>DLSSLTPGGSMGLQVNRGSQSSLEGAPATAPEPHSLGILHASYSVSHRVRPWWDITSCRQQWTRQILKDVSLYVESGQIMCILGSSGSGKTTLLDAMSGRLGRAGTFLGEVYVNGRALRREQFQDCFSYVLQSDTLLSSLTVRETLHYTALLAIRRGNPGSFQKKVEAVMAELSLSHVADRLIGNYSLGGISTGERRRVSIAAQLLQDPKVMLFDEPTTGLDCMTANQIVVLLVELARRNRIVVLTIHQPRSELFQLFDKIAILSFGELIFCGTPAEMLDFFNDCGYPCPEHSNPFDFYMDLTSVDTQSKEREIETSKRVQMIESAYKKSAICHKTLKNIERMKHLKTLPMVPFKTKDSPGVFSKLGVLLRRVTRNLVRNKLAVITRLLQNLIMGLFLLFFVLRVRSNVLKGAIQDRVGLLYQFVGATPYTGMLNAVNLFPVLRAVSDQESQDGLYQKWQMMLAYALHVLPFSVVATMIFSSVCYWTLGLHPEVARFGYFSAALLAPHLIGEFLTLVLLGIVQNPNIVNSVVALLSIAGVLVGSGFLRNIQEMPIPFKIISYFTFQKYCSEILVVNEFYGLNFTCGSSNVSVTTNPMCAFTQGIQFIEKTCPGATSRFTMNFLILYSFIPALVILGIVVFKIRDHLISRGSHHHHHHGHHHHHH[2x];>MGSAGKAAEERGLPKGATPQDTSGLQDRLFSSESDNSLYFTYSGQPNTLEVRDLNYQVDLASQVPWFEQLAQFKMPWTSPSCQNSCELGIQNLSFKVRSGQMLAIIGSSGCGRASLLDVITGRGHGGKIKSGQIWINGQPSSPQLVRKCVAHVRQHNQLLPNLTVRETLAFIAQMRLPRTFSQAQRDKRVEDVIAELRLRQCADTRVGNMYVRGLSGGERRRVSIGVQLLWNPGILILDEPTSGLDSFTAHNLVKTLSRLAKGN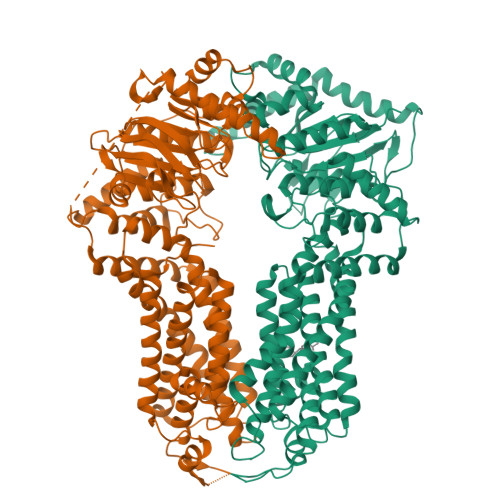RLVLISLHQPRSDIFRLFDLVLLMTSGTPIYLGAAQHMVQYFTAIGYPCPRYSNPADFYVDLTSIDRRSREQELATREKAQSLAALFLEKVRDLDDFLWKAETKDLDEDTCVESSVTPLDTNCLPSPTKMPGAVQQFTTLIRRQISNDFRDLPTLLIHGAEACLMSMTIGFLYFGHGSIQLSFMDTAALLFMIGALIPFNVILDVISKCYSERAMLYYELEDGLYTTGPYFFAKILGELPEHCAYIIIYGMPTYWLANLRPGLQPFLLHFLLVWLVVFCCRIMALAAAALLPTFHMASFFSNALYNSFYLAGGFMINLSSLWTVPAWISKVSFLRWCFEGLMKIQFSRRTYKMPLGNLTIAVSGDKILSVMELDSYPLYAIYLIVIGLSGGFMVLYYVSLRFIKQKPSQDWASNSLEVLFQME[2x]>[4x]MSLDRVDWPHATFSTPVKRIFDTQTTLDFQSSLAIHRIKYHLHKYTTLISHCSDPDPHAT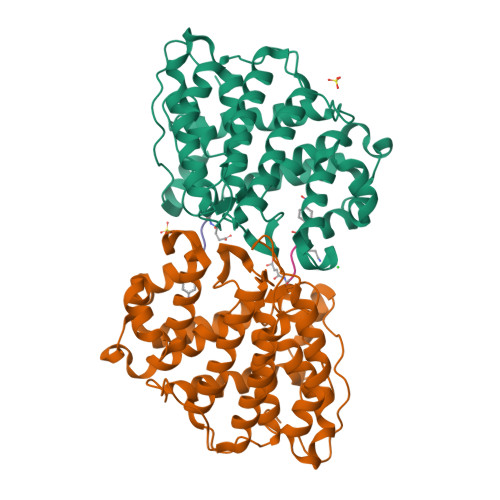ASSIAMVNGLMGVLDKLAHLIDETPPLPGPRRYGNLACREWHHKLDERLPQWLQEMLPSEYHEVVPELQYYLGNSFGSSTRLDYGTGHELSFMATVAALDMLGMFPHMRGADVFLLFNKYYTIMRRLILTYTLEPAGSHGVWGLDDHFHLVYILGSSQWQLLDAQAPLQPREILDKSLVREYKDTNFYCQGINFINEVKMGPFEEHSPILYDIAVTVPRWSKVCKGLLKMYSVEVLKKFPVVQHFWFGTGFFPWVNIHHHHHH> GSHMSTGDFLTKGIELVQKAIDLDTATQYEEAYTAYYNG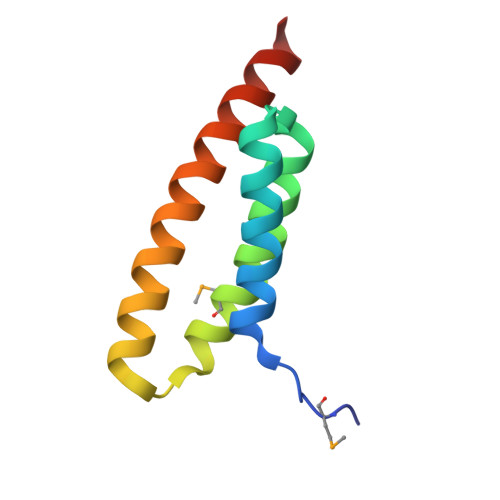LDYLMLALKYEKNPKSKDLIRAKFTEYLNRAEQLKKHLESEEANAA>MKLSPKAATLAERSAGLAFSLYQAMAKDQAVENILLSPVVVASSLGLVSLGGKATTASQAKAVLSAEQLRDEEVHAGLGELLRSLSNSTARNVTWKLGSRLYGPSSVSFAEDFVRSSKQHYNCEHSKINFRDKRSALQSINEWAAQTTDGKLPEVTKDVERTDGALLVNAMFFKPHWDEKFHHKMVDNRGFMVTRSYTVGVTMMHRTGLYNYYDDEKEKLQIVEMPLAHKLSSLIILMPNNVEPLERLEKLLTKEQLKIWMGKMQKKAVAISLPKGVVEVTHDLQKHLAGLGLTEAIDKNKADLSRMSGKKDLYLASVFHATAFEWDTEGNPFDQDIYGREELRSPKLFYADHPFIFLVRDTQSGSLLFIGRLVRPKGDKMRDELLEHHHHHH[4x];>[6x]XPPGPPGPRGPPGPPGX

In order to function, collagens require the specific chaperone HSP47 for proper folding and secretion. Proper triple-helix formation as well as exit from the ER of procollagen molecules depends critically on HSP47, an ER-resident chaperone belonging to the serpin family. The interaction involves Gly-Xxx-Arg triplets exclusively on triple-helical procollagen. The arginine residue is located in the so-called Y0 position and forms a crucial salt bridge with an aspartic acid of HSP47 (16).

While homotrimeric procollagen molecules, therefore, always expose three potential binding sites per such a triplet, so far invariably a 2:1 HSP47:triple-helix stoichiometry has been found. In these complexes, the two HSP47 molecules bind to the leading and trailing strand of the triple helix, while the binding site of the middle strand remains unoccupied due to steric reasons. In all our previous HSP47 cocrystal structures with homotrimeric RGP motifs, the arginine residues on the trailing and leading strand each bound to one HSP47 molecule. There is no space for a third HSP47 molecule on the middle strand of the collagen triple helix. Exactly this configuration is also seen in a hitherto unpublished structure of the HSP47 double-mutant H273N/H274N, which exhibits a decreased dissociation rate off collagen at low pH. Although the complex of this mutant with the collagen model peptide Ac-(PPG)2PTGPRG(PPG)2-NH2 crystallizes in space group P21, which also has not been observed in any other HSP47 crystal form so far, its structure is virtually indistinguishable from the other structures of HSP47 in complex with various collagen RGP model peptides of different length.>[2x]MSLVLNFVGTGTLTRFFLECLKDRYEIGYILSRSIDRARNLAEVYGGKAATLEKHPELNGVVFVIVPDRYIKTVANHLNLGDAVLVHCSGFLSSEIFKKSGRASIHPNFSFSSLEKALEMKDQIVFGLEGDERGLPIVKKIAEEISGKYFVIPSEKKKAYHLAAVIASNFPVALAYLSKRIYTLLGLDEPELLIHTLMKGVADNIKKMRVECSLTGPVKRGDWQVVEEERR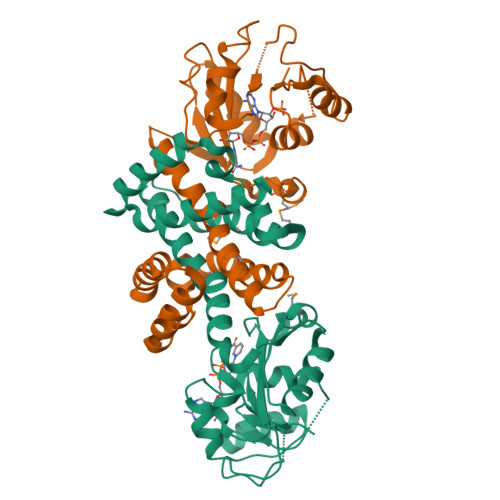EYEKIFGNTVLYDEIVKLLREVAESERREAQEDEREGGSHHHHHH N-[(6-BUTOXYNAPHTHALEN-2-YL)SULFONYL]-L-GLUTAMIC ACID | C19 H23 N O7 S | 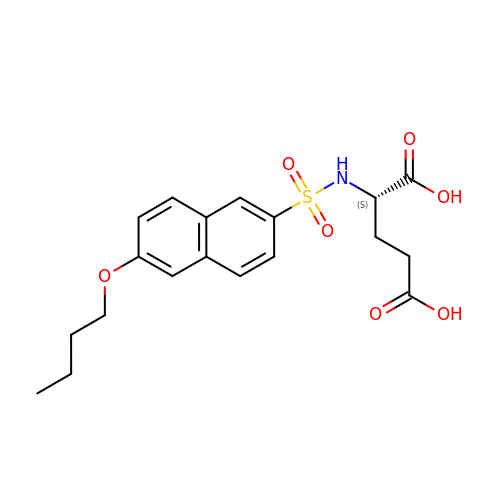UAGYXJBYAFGRFR-KRWDZBQOSA-N>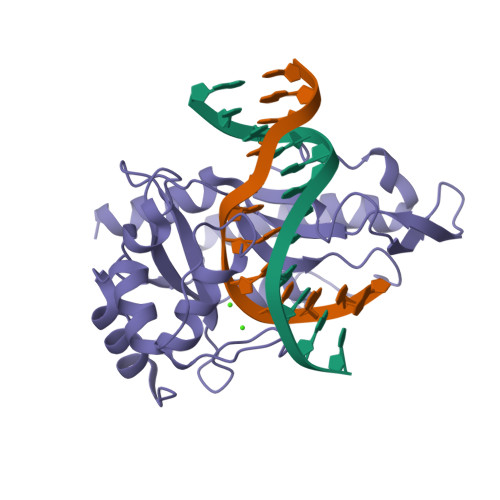 MIPQTLEQLLSQAQSIAGLTFGELADELHIPVPIDLKRDKGWVGMLLERALGATAGSKAEQDFSHLGVELKTLPINAEGYPLETTFVSLAPLVQNSGVKWENSHVRHKLSCVLWMPIEGSRHIPLRERHIGAPIFWKPTAEQERQLKQDWEELMDLIVLGKLDQITARIGEVMQLRPKGANSRAVTKGIGKNGEIIDTLPLGFYLRKEFTAQILNAFLETKSL BETA-L-ASPARTIC ACID | C4 H7 N O4 | 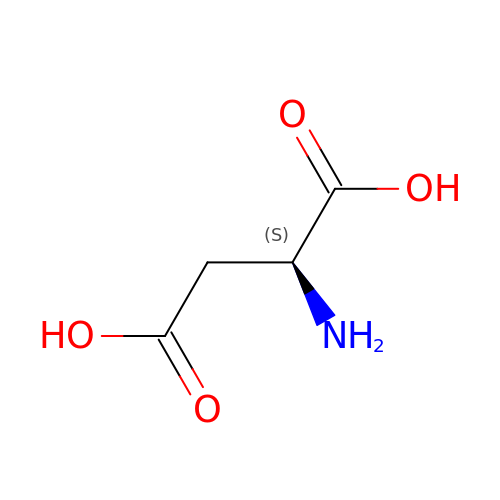CKLJMWTZIZZHCS-REOHCLBHSA-N>SMDDSETGFNLKVVLVSFKQCLDEKEEVLLDPYIASWKGLVRFLNSLGTIFSFISKDVVSKLRIMERLRGGPQSEHYRSLQAMVAHELSNRLVDLERRSHHPESGCRTVLRLHRALHWLQLFLEGLRTSPEDARTSALCADSYNASLAAYHPWVVRRAVTVAFCTLPTREVFLEAMNVGPPEQAVQMLGEALPFI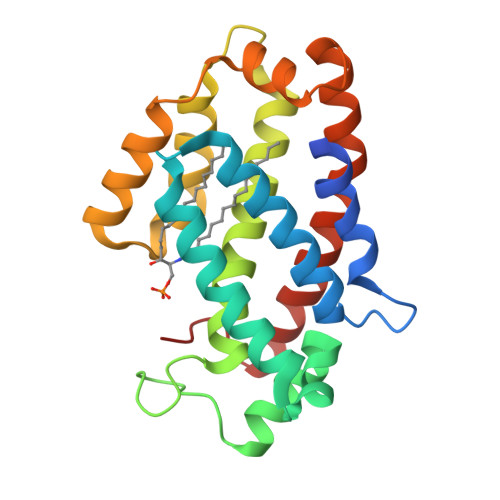QRVYNVSQKLYAEHSLLDLP[2x]>GAAGKRARAKRATKSGKDSALAPKIAPPVPTCGITTYSPPTDGSCGWHVLAAIVNRMINGDFTSPLPQYNRPEDDWASDYDLAQAIQCLQLPATVVRNRACPNAKYLIKLNGVHWEVEVRSGMAPRSLSRECVVGVCSEGCVAPPYPADGLPKRALEALASAYRLPSDCVSSGIADFLADPPPQEFWTLDKMLTGSSGHHHHHH[2x]

PRRSV replication is accomplished with the help of four virus-encoded proteases–one of which is the papain-like protease 2 (PLP2), located within nsp2, which processes the nsp2|3 cleavage site to release nsp2 from the rest of the viral polyprotein. Subsequent work demonstrated that several arterivirus OTU domain proteases hydrolyze ubiquitin (Ub) thereby downregulating Ub-dependent cellular innate immune signaling pathways as means to evade host antiviral mechanisms. To this end, we determined the crystal structure of the PRRSV PLP2 domain both in the presence and absence of its Ub substrate to a resolution of 2.85Å and 2.3Å, respectively. Overall, PLP2 adopts a similar, compact OTU-like fold similar to that of the previously determined EAV PLP2 domain, comprising of α and β lobes, as well as a structural 4-cysteine zinc finger, and a DALI search indicates the PRRSV PLP2 domain most closely resembles that of EAV PLP2.

To begin characterization of the PRRSV PLP2 domain structure, we determined the crystal structure of the enzyme from PRRSV Type I strain SD01-08. The SD01-08 PLP2 domain crystallized in space group C2221, with 2 copies present in the asymmetric unit. The 2 copies superposed with an RMSD of 0.635 Å over 144 Cα atoms, with unremarkable differences between the structures. Residues 385–415, representing the N-terminus of nsp2 following polyprotein cleavage were not visible in electron density maps. In particular, the α-helical lobe of the PRRSV PLP2 is comprised of a 4-helix bundle as opposed to a 3-helix bundle seen in EAV PLP2. The PRRSV PLP2 active site however is made up of a catalytic dyad formed by C429 and H498 and lacks an obvious third coordinating residue. Additionally, in the apo structure, H498 is positioned away from C429 in a catalytically incompetent conformation. Although unusual, similar active site conformations have been characterized in the OTU DUBs Cezanne, OTULIN, Gumby, OTUB1 and TYMV PRO. Structural regions surrounding the active site of PRRSV PLP2 show a high degree of mobility, as evidenced by higher B-factors in these areas. These regions include the β3-β4 loop (residues 493–499) which contains H498, the 453 loop which extends toward helix α2, an active site loop (residues 422–428) extending towards the catalytic C429, which also forms the oxyanion hole, and the 480 loop situated near the Ub-binding region.> KPEFDPILLRPVD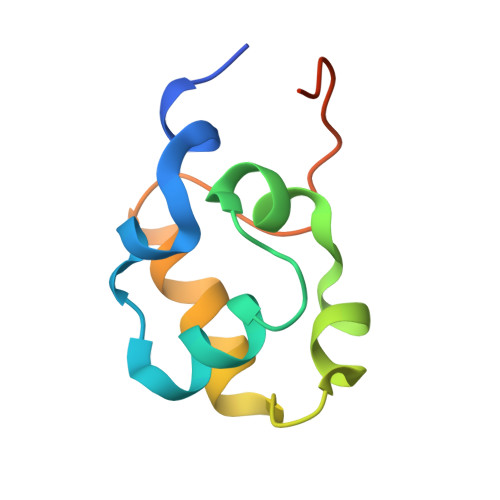DLELTVRSANCLKAEAIHYIGDLVQRTEVELLKTPNLGKKSLTEIKDVLASRGLSLGMRLENWPPASIADE>[2x]MAGSYNYAEALQKAIYFYECQQAGPLPEWNRVEWRGDATMNDEVLGGWYDAGDHVKFNLPMAYSAAMLGWALYEYGDDIEASGQRLHLERNLAFALDYLVACDRGDSVVYQIGDGAADHKWWGSAEVIEKEMTRPYFVGKGSAVVGQMAAALAVGSIVLKNDTYLRYAKKYFELADATRSDSTYTAANGFYSSHSGFWDELLWASTWLYLATGDRNYLDKAESYTPKLNRQNQTTDIEYQWAHCWDDCHYGAMILLARATGKEEYHKFAQMHLDWWTPQGYNGKRVAYTPGGLAHLDTWGPLRYATTEAFLAFVYADSINDPALKQKYYNFAKSQIDYALGSNPDN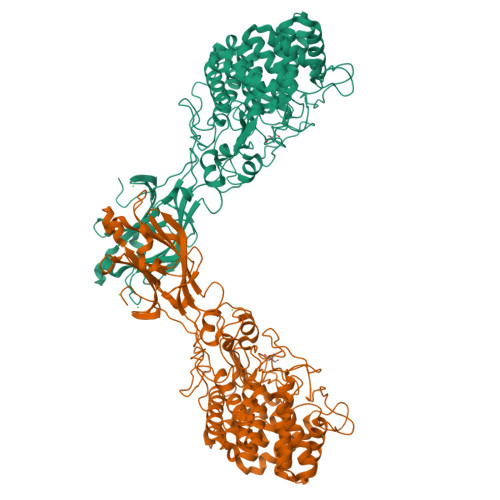RSYVVGFGNNPPQRPHHRTAHGTWLDKRDIPEKHRHVLYGALVGGPGRDDSYEDNIEDYVKNEVACDYNAGFVGALCRLTAEYGGTPLANFPPPEQRDDEFFVEAAINQASDHFTEIKALLNNRSSWPARLIKDLSYNYYMDLTEVFEAGYSVDDIKVTIGYCESGMDVEISPITHLYDNIYYIKISYIDGTNICPIGQEQYAAELQFRIAAPQGTKFWDPTNDFSYQGLTRELAKTKYMPVFDGATKIFGEVPGGLEHHHHHH> MHHHHHHHHENLYFQGGSSTAGDPTAKLVRLNPRGGDGPGIVFAPPAGGTVLGYIELARHLKGFGEIHGVEAPGLGAGETPVYPSFEEMVQFCSDSAAGVAGDGVYIGGHALGGHIAFYLATMLLDRGIRPKGLIILDTPPRLGDIPVADADLTEEETKVFILAMGIGGMLDQDRDALKDLPYEE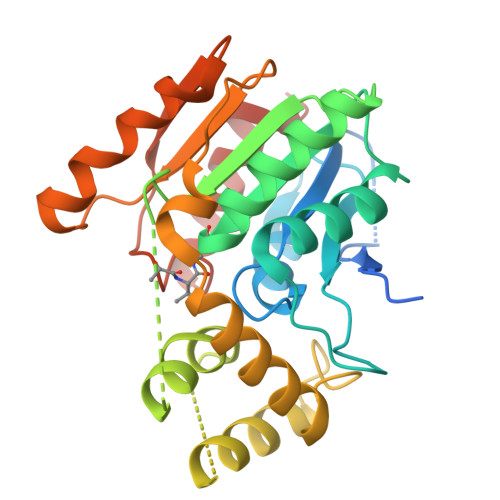AKQLLLDRAKNDPRVSAFLSEDYLDRFLRLQMHQLMYSRDVVLPQRKLDIPIHVFRTKNHAPEVARLFSAWENYAAGEVTFVDIPGDHATMLRAPHVSEVAQLLDRHCGLPSDDGPRG>GHHHHHHVPAFLTKLWTLVSDPDTDALICWSPSGNSFHVFDQGQFAKEVLPKYFKHNNMASFVRQLNMYGFRKVVHIEQGGLVKPERDDTEFQHPCFLRGQEQLLENIK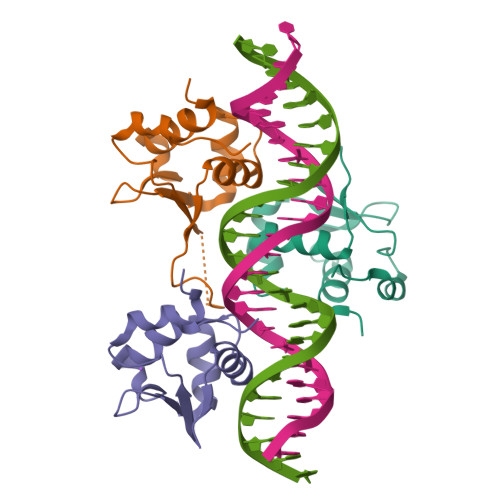RKVT[6x]>[2x]SMDPERRVRSTLKKVFGFDSFKTPLQESATMAVVKGNKDVFVCMPTGAGKSLCYQLPALLAKGITIVVSPLIALIQDQVDHLLTLKVRVSSLNSKLSAQERKELLADLEREKPQTKILYITPEMAASSSFQPTLNSLVSRHLLSYLVVDEAHCVSQWGHDFRPDYLRLGALRSRLGHAPCVALTATATPQVQEDVFAALHLKKPVAIFKTPCFRANLFYDVQFKELISDPYGNLKDFCLKALGQEADKGLSGCGIVYCRTREACEQLAIELSCRGVNAKAYHAGLKASERTLVQNDWMEEKVPVIVATISFGMGVDKANVRFVAHWNIAKSMAGYYQESGRAGRDGKPSWCRLYYSRNDRDQVSFLIRKEVAKLQEKRGNKASDKATIMAFDALVTFCEELGCRHAAIAKYFGDALPACAKGCDHCQNPTAVRRRLEALERSSSWSKTCIGPSQGNGFDPELYEGGRKGYGDFSRYDEGSGGSGDEGRDEAHKREWNLFYQKQMQLRKGKDPKIEEFV

RECQL5 (also known as RECQ5) is a member of the RecQ family of helicases, which are highly conserved throughout evolution, and function in many diverse cellular processes with the role of maintaining genome integrity. Specific roles have been established for RECQL5 in almost every cellular process involving DNA, including transcription, replication, recombination, chromosomal segregation and DNA repair. The Zn2+-binding domain consists of a pair of long antiparallel α-helices (also known as the helical hairpin), followed by series of short helices and loops, from which a cluster of cysteine residues bind in a typical Cys4 tetrahedral arrangement to a single Zn2+ ion.

Crystals of the Apo form of RECQL5 were obtained using a construct spanning residues 11–526, this includes both D1 and D2 RecA like domains, the Zn2+ binding subdomain, and a short section (residues 438–453) of the previously uncharacterized RECQL5 C-terminal region. Crystals were obtained for the APO protein which diffracted to a maximum resolution of 3.2 Å, and the structure was solved by molecular replacement using the structure of BLM helicase as a search model, with two chains in the asymmetric unit. The model is complete from residues 12–452, with the exception of loops 250–260 and 321–323 which could not be modeled due to disorder. The final 74 residues at the C-terminus are absent from the model, and appear to be completely disordered from the electron density maps, indicating this region is disordered, consistent with the results of various disorder prediction servers. The most prominent difference is in the relative orientations of the D1 and D2 domains, with the inter-domain cleft almost completely closed in the APO form and considerably more open in the ADP bound form, with maximal displacements of equivalent residues of up to 30 Å. Similarly, the ‘closed’ APO structures cluster at the bottom of the plot with RECQL5 being similar to the APO form of E. coli RecQ, and chain B of APO D. radiodurans RecQ (chain A is in a rather more open state). Comparisons with other RecQ family structures show the ‘closed’ APO form to be more typical of the conformation found in other structures, while solution studies show that the ‘open’ ADP form predominates in solution. The APO form is believed to bind to DNA primarily via D2, with motif VI forming polar contacts to the AR loop stabilizing the low affinity state. Finally following ADP release the relatively long range charge interactions between the acidic residues on motif II and the basic residues on motif IV (which are no longer shielded by the nucleotide or magnesium ions), would bring the two domains close together to form the closed conformation again.>[30x]MESKALLLLALSVCLQSLTVSRGGLVAADRITGGKDFRDIESKFALRTPEDTAEDTCHLIPGVTESVANCHFNHSSKTFVVIHGWTVTGMYESWVPKLVAALYKREPDSNVIVVDWLSRAQQHYPVSAGYT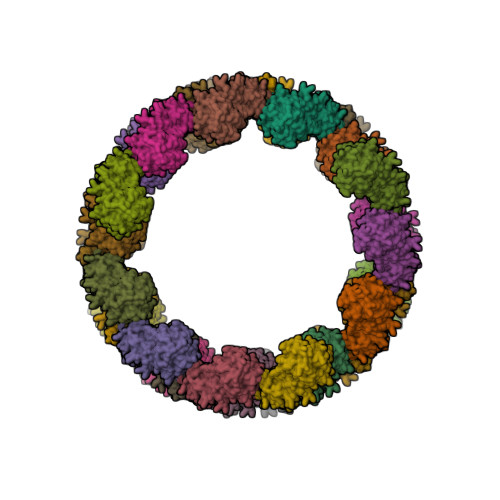KLVGQDVAKFMNWMADEFNYPLGNVHLLGYSLGAHAAGIAGSLTNKKVNRITGLDPAGPNFEYAEAPSRLSPDDADFVDVLHTFTRGSPGRSIGIQKPVGHVDIYPNGGTFQPGCNIGEALRVIAERGLGDVDQLVKCSHERSVHLFIDSLLNEENPSKAYRCNSKEAFEKGLCLSCRKNRCNNMGYEINKVRAKRSSKMYLKTRSQMPYKVFHYQVKIHFSGTESNTYTNQAFEISLYGTVAESENIPFTLPEVSTNKTYSFLLYTEVDIGELLMLKLKWISDSYFSWSNWWSSPGFDIGKIRVKAGETQKKVIFCSREKMSYLQKGKSPVIFVKCHDKSLNRKSG> PISPIETVPVKLKPGMDGPKVKQWPLTEEKIKALVEICTEMEKEGKISKIGPENPYNTPVFAIKKKDSTKWRKLVDFRELNKRTQDFWEVQLGIPHPAGLKKKKSVTVLDVGDAYFSVPLDEDFRKYTAFTIPSINNETPGIRYQYNVLPQGWKGSPAIFQSSMTKILEPFRKQNPDIVIYQYMDDLCVGSDLEIGQHRTKIEELRQHL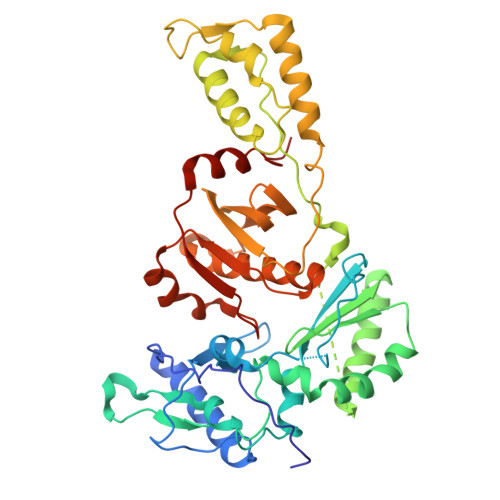LRWGLTTPDKKHQKEPPFLWMGYELHPDKWTVQPIVLPEKDSWTVNDIQKLVGKLNWASQIYPGIKVRQLCKLLRGTKALTEVIPLTEEAELELAENREILKEPVHGVYYDPSKDLIAEIQKQGQGQWTYQIYQEPFKNLKTGKYARMRGAHTNDVKQLTEAVQKITTESIVIWGKTPKFKLPIQKETWETWWTEYWQATWIPEWEFVNTPPLVKLWYQLEKEPIVGAETF>MHRTYSLRNSRAPTASQLQNPPPPPSTTKGRFFGKGGLAYSFRRSAAGAFGPELSRKLSQLVKIEKNVLRSMELTANERRDAAKQLSIWGLENDDDVSDITDKLGVLIYEVSELDDQFIDRYDQYRLTLKSIRDIEGSVQPSRDRKDKITDKIAYLKYKDPQSPKIEVLEQELVRAEAESLVAEAQLSNITRSKLRAAFNYQFDSIIEHSEKIALIAGYGKALLELLDDSPVTPGETRPAYDGYEASKQIIIDAESALNEWTLDSAQVKPTLSFKQDYEDFEPEEGEEEEEEDGQGRWSEDEQEDGQIEEPEQEE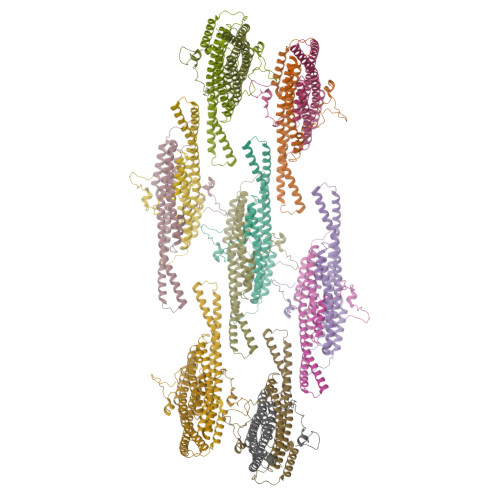EGAVEEHEQVGHQQSESLPQQTTA[14x]>MRGSHHHHHHGSLSSSPSEILQELGKGSTHPQPGVSPPAAPAAPGPKDGPGETDAFGNSEGKELVASGENKIKQGLLPSLEDLLFYTIAEGQEKIPVHKFITALKSTGLRTSDPRLKECMDMLRLTLQTTSDGVMLDKDLFKKCVQSNIVLLTQAFRRKFVIPDFMSFTSHIDELYESAKKQSGGKVADYIPQLAKFSPDLWGVSVCTVDGQRHSTGDTKVPFCLQSCVKPLKYAIAVNDLGTEYVHRYVGKEPSGLRFNKLFLNEDDKPHNPMVNAGAIVVTSLIKQGVNNAEKFDYVMQFLNKMAGNEYVGFSNATFQSERESGDRNFAIGYYLKEKKCFPEGTDMVGILDFYFQLCSIEVTCESASVMAATLANGGFCPITGERVLSPEAVRNTLSLMHSCGMYDFSGQFAFHVGLPAKSGVAGGILLVVPNVMGMMCWSPPLDKMGNSVKGIHFCHDLVSLCNFHNYDNLRHFAKKLDPRREGGDQR[4x]

Cancer cells often overexpress glutaminase enzymes, in particular glutaminase C (GAC), which resides in the mitochondria and catalyzes the hydrolysis of glutamine to glutamate. Glutamate is then either used to fuel the TCA cycle via its conversion to α-ketoglutarate by glutamate dehydrogenase or as a building block for various biomolecules. Numerous GAC inhibitors have been reported, with the most heavily investigated being a class of compounds derived from the small molecule bis-2-(5-phenylacetamido-1,3,4-thiadiazol-2-yl)ethyl sulfide (BPTES). These compounds bind at the dimer/dimer interface of the GAC tetramer, which is near the so-called activation loop (Gly315 to Glu325), effectively trapping the tetrameric enzyme in an inactive conformation.

However, the serial room temperature structure for the GAC–BPTES complex shows that one of the two BPTES molecules assumes a more extended orientation compared to UPGL00004, whereas in the cryo-cooled co-crystal structure of GAC bound to BPTES, each of the two bound BPTES molecules adopt an orientation similar to UPGL00004. The extension of the BPTES molecule in the serial room temperature structure is most dramatically demonstrated by the distance between its terminal rings. In this case, the ring-to-ring distance is 18.5 Å, which is significantly larger than the distances between the rings in either the cryo-cooled structure (14.4 Å) or for the UPGL0004 molecule (14.6 Å in the cryo-cooled structure and 14.7 Å in the room-temperature structure). In fact, the BPTES molecule in the serial room temperature structure also shows the highest B-factor, suggesting that that the weaker inhibitor (BPTES) undergoes multiple conformational changes before stabilizing in the cup-like orientation as always observed for UPGL0004. Examining the interactions with the activation loop reveals that the thiadiazole ring within the more linear end of the extended BPTES molecule in the room temperature structure for the GAC–BPTES complex is shifted away from its hydrogen bonding partner, the backbone NH of Phe 322 (4.3 Å distance for the more-linear end versus 3.8 Å for the more cup-shaped end of the molecule). This apparent disruption of hydrogen bonds between GAC and the thiadiazole ring in BPTES, compared to the same ring in UPGL00004 (3.7 Å distance), might partially explain the basis for BPTES having a weaker binding affinity and lower potency with GAC.>MAKDKEFQVLFVLTILTLISGTIFYSTVEGLRPIDALYFSVVTLTTVGDTPPPQTDFGKIFTILYIFIGIGLVFGFIHKLAVNVQLPSILS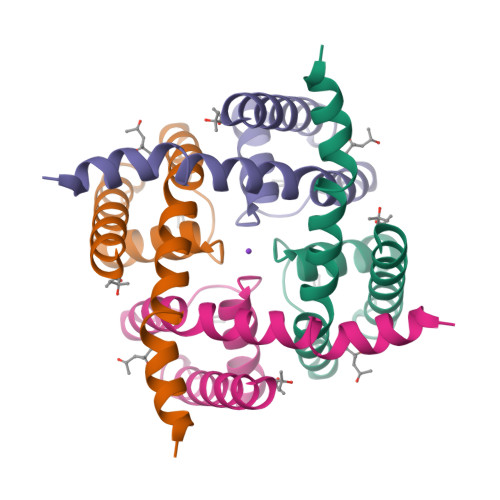NLVPR[2x]>MFEARLVQGSILKKVLEALKDLINEACWDISSSGVNLQSMDSSHVSLVQLTLRSEGFDTYRCDRNLAMGVNLTSMSKILKCAGNEDIITLRAEDNADTLALVFEAPNQEKVSDYEMKLMDLDVEQLGIPEQEYSCVVKMPSGEFARICRDLSHIGDAVVISCAKDGVKFSASGELGNGNIKLSQTSNVDKEEEAVTIEMNEPVQLTFALRYLNFFTKATPLSSTVTLIMSADVPLVVEYKIADMGHLKYYLAPKIEDE[3x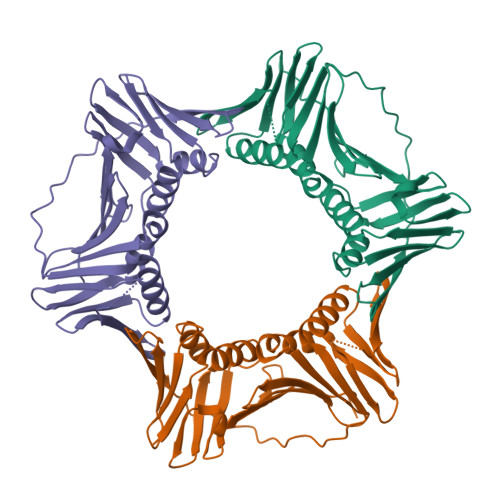]> GARASVLSGGELDKWEKIRLRPGGKKQYKLKHIVWASRELERFAVNPGLLETSEGCRQILGQLQPSLQTGSEELRSLYNTIAVLYCV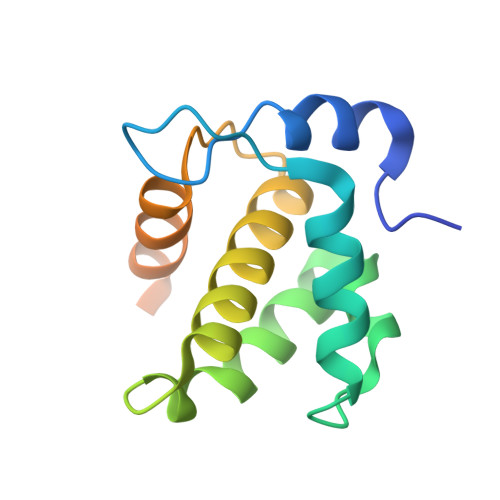HQRIDVKDTKEALDKIEEEQNKSKKKAQQAAADTGNNSQVSQNY> SHGELTPDQQTLLHFIMDSYNKQRMPQEITNKILKEEFSAEENFLILTEMATNHVQVLVEFTKKLPGFQTLDHEDQIALLKGSAVEAMFLRSAEIFNKKLPSGHSDLLEERIRNSGISDEYITP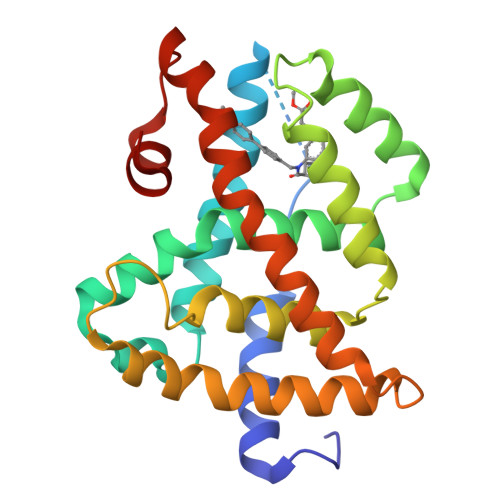MFSFYKSIGELKMTQEEYALLTAIVILSPDRQYIKDREAVEKLQEPLLDVLQKLCKIHQPENPQHFACLLGRLTELRTFNHHHAEMLMSWRVNDHKFTPLLCEIWDVQ>MVEIKLENIVKKFGNFTALNNINLKIKDGEFMALLGPSGSGKSTLLYTIAGIYKPTSGKIYFDEKDVTELPPKDRNVGLVFQNWALYPHMTVYKNIAFPLELRKAPREEIDKKVREVAKMLHIDKLLNRYPWQLSGGQQQRVAIARALVKEPEVLLLDEPLSNLDALLRLEVRAELKRLQKELGITTVYVTHDQAEALAMADRIAVIREGEILQVGTPDEVYYKPKYKFVGGFLGNPPMNFVEAKVEDGKLVITEKSKLPIPKQYVEIVKETGITEVIIGFRPHDAEIVKGEGEGIVGEVYSFEPLGREQIVTVSVNDSIVKVFAPEGEHFSFGEK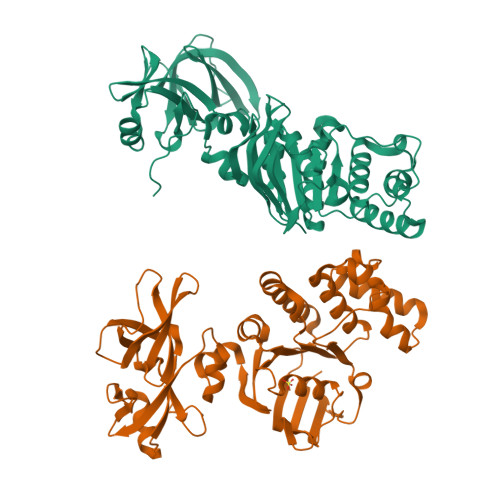VTIKVKEELLVLFDKKTEKALEFSKL[2x]> AKCDDGRTTANAA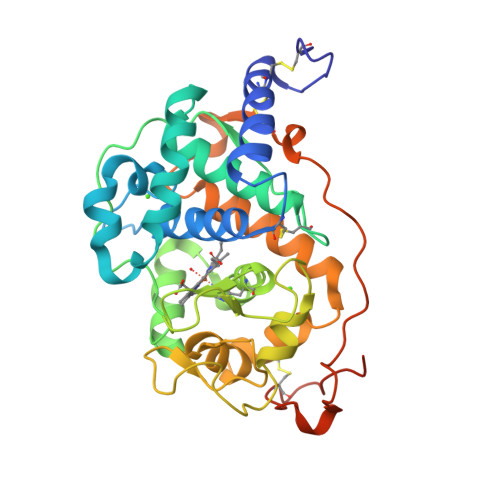CCILFPILDDIQENLFDGAQCGEEVHESLRLTFHDAIGFSPTLGGGGADGSIIAFSDIETNFPANAGIDEIVEAQKPFVAKHNISAGDFIQFAGAVGVSNCPGGVRIPFFLGRPDAVKASPDHLVPEPFDSVTSILARMGDAGFSPVEVVWLLASHSIAAADKVDPSIPGTPFDSTPGVFDSQFFIETLLKGRLFPGTADNKGEAKSPLQGEIRLQSDELLARDPRTACEWQSMVNNQPKIQNRFAATMSKMALLGQDKTKLIDCSDVIPTPPARVGAAHLPAGFSLKDVEQACRKTPFPRLTADPGPVTSVPPVPGS> GLFDAPGRSQFVPADQAFAFDFQQNQHDLNLTWQIKDGYYLYRKQIRITPEHAKIADVQLPQGVWHEDEFYGKSEIYRDRLTLPVTINQASAGATLTVTYQGAA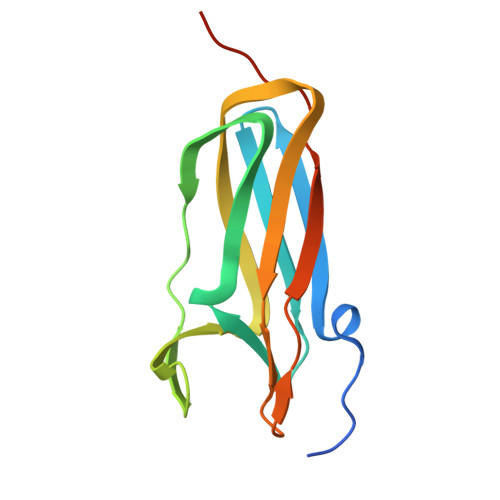DAGFCYPPETKTVPLSEVVANNAAPQPV> SN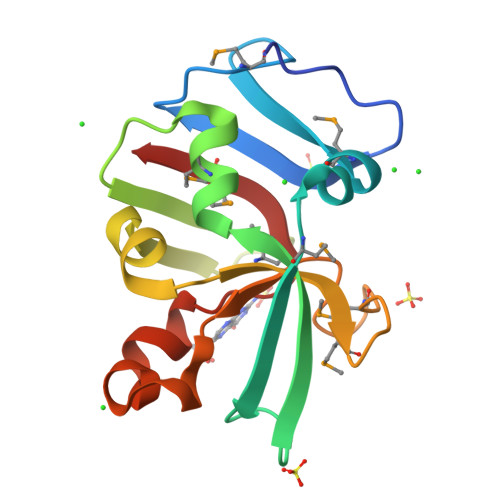AEKLPAPTGKPVLTISGKIGNMNVGDKAVFDLAMLEKLGMKTIETTTPWYTGKVRFDGIPLNKLMDLVGAKGTSARVLALNDYTTIIPIDDFYKFPVIMALKMNGQYMRIRDKGPLFIVYPYDSSAELQNQIYYSRSAWQVSKMIIE>MTDQTTVVDITSAPLTPKEKLDLYCEALCDGFNKTQAYIKAGFSAPHAQRNVAPYHRKNAEYIQAYISERIGSDAPAARKVVLEIMNDPNEKGGIRLKAAQDILDRAGFGAKQKIELTTKDVADLTTEDIKNELAKLFNDEPELAKVVAFPINHSKS[81x]

The genome packaging motor of tailed bacteriophages and herpesviruses is a powerful nanomachine built by several copies of a large (TerL) and a small (TerS) terminase subunit. In contrast, TerS is a DNA recognition subunit that binds packaging initiation sites (referred to as pac or cos) in preparation for genome packaging. TerS also stimulates the ATPase activity of TerL, while repressing the large terminase nuclease activity. Thus, three related small terminase subunits from Pseudomonas phages PaP3, NV1 and LUZ24 are polymorphic in solution but adopt a nonameric quaternary structure in the high affinity heparin-binding conformation.

NV1 TerS crystallized in a large monoclinic unit cell with five nonamers in the AU that diffracted weakly to 3.95 Å resolution. The structure of NV1 TerS was then solved by MR using the model of PaP3 TerS and refined to an Rwork/Rfree of 25.9/29.1% at 3.95 Å resolution, enforcing 81-fold NCS torsion restraints. NV1 and PaP3 TerSs are virtually identical (RMSD ∼ 1.1), as expected for two proteins that are ∼65% identical in amino acid sequence. Peak 1 and peak 2 had a roughly equal quantity of protein for PaP3 and LUZ24, whereas most of NV1 TerS eluted in peak 2. The same intramolecular plasticity observed in PaP3 likely exists in the TerSs from NV1 and LUZ24. SEC-SAXS of PaP3 and NV1 TerS revealed a radius of gyration (Rg) of 41.44 ± 0.40 Å and 41.33 ± 0.43 Å, respectively,, which is larger than the calculated crystal structure Rg values of 33.84 Å and 33.32 Å, respectively. The distance distribution function P(r) calculated from SAXS data indicates a maximum diameter Dmax ∼131 Å for both PaP3 and NV1 TerS, also about 25% larger than the maximum width of the crystal structure (∼105 Å). Similarly, the NV1 TerS crystal structure docked into the 9-fold electron SAXS density revealed modest agreement between solution and crystal structure (χ2 = 2.55), despite the exceptional quality of this SAXS density. In both cases, the solution structure of TerS had a wider outer diameter than the crystal structure and showed extra density for the missing C-terminal tail. In contrast, using 10- or 8-fold rotational symmetry did not significantly improve the FSC resolution, supporting the notion PaP3 and NV1 TerSs exist in solution as nonamers.Whereas previous studies on salivary gland extracts from the sandfly Lutzomyia longipalpis identified SALO (salivary anticomplement from L. longipalpis) as a potent inhibitor of the classical complement pathway (CP), its precise mechanism of action has remained elusive. We found that SALO inhibits the CP by binding specifically to the zymogen form of C1r. We provide two crystal structure determinations and supporting functional studies which show that SALO binds tightly to the zymogen activation loop of C1r preventing cleavage of its scissile bond. However, since the C1r zymogen undergoes autoactivation over time, we expressed an engineered fragment of human C1r consisting of its two CCP repeats and its serine protease domain, wherein the catalytic serine (S654) had been mutated to alanine (zC1r-12SP).

Thereafter, we crystallized eSALO-WT bound to zC1r-12SP, collected X-ray diffraction data extending to 3.3 Å limiting resolution, and solved the structure by molecular replacement. The asymmetric unit of the crystal contained two copies of the eSALO-WT–zCr-12SP complex, which superimposed well upon each other (RMSD = 0.34 Å across 444 equivalent Cα positions); thus, our subsequent analyses focused on the eSALO-WT–zC1r-12SP complex represented by chains A and C. Whereas the eSALO-WT–zC1r-12SP interaction buried ∼1100 Å2 of surface area at the interface, the most extensive interactions between the two proteins were centered upon the zymogen activation loop of zC1r-12SP. By contrast, there were no contacts between eSALO-WT and either of the CCP domains of the protease, which may be less accessible within the context of the larger C1 structure. Consistent with this, EBI-PISA identified 13 likely hydrogen bonds and four candidate salt bridges between the residues lining this channel, including N33 and Y/X51 (explained further in the following subsection), and residues from the zymogen activation loop of zC1r-12SP, which is composed roughly of residues V458-Q468 inclusive. At the periphery of the eSALO-WT channel, the side chain of E58 formed a salt bridge with the side chain of R461 from zC1r-12SP. Finally, outside the concave channel, residues on the first α helix of eSALO-WT, including D32, appeared to contact a secondary site on zC1r-12SP, which is composed of residues H642–Q647 inclusive. During the course of model building and refinement, we noticed a strong, positive feature in the Fo–Fc electron density map distal to the hydroxyl group of eSALO-WT residue Y51. Based on the geometry of this electron density, we suspected that Y51 had undergone post-translational sulfation during eSALO-WT expression and secretion from HEK293(T) cells. Therefore, we subsequently modeled this residue as sulfotyrosine, X51. In the final model, this sulfate group formed three different hydrogen bonds ranging from 2.6 to 3.2 Å in length with groups derived from R463 and I464, which are the two residues linked by the scissile bond in the C1r zymogen.

>SEDCENIFHDNAYLLKLDCEAGRVDPVEYDDISDEEIYEITVDVGVSSEDQEKVAKIIRECIAQVSTQDCTKFSEIYDCYMKKKICNYYPENMGSGHHHHHHHH[2x];>KCPQPKTLDEFTIIQNLQPQYQFRDYFIATCKQGYQLIEGNQVLHSFTAVCQDDGTWHRAMPRCKIKDCGQPRNLPNGDFRYTTTMGVNTYKARIQYYCHEPYYKMQTRAGSRESEQGVYTCTAQGIWKNEQKGEKIPRCLPVCGKPVNPVEQRQRIIGGQKAKMGNFPWQVFTNIHGRGGGALLGDRWILTAAHTLYPKEHEAQSNASLDVFLGHTNVEELMKLGNHPIRRVSVHPDYRQDESYNFEGDIALLELENSVTLGPNLLPICLPDNDTFYDLGLMGYVSGFGVMEEKIAHDLRFVRLPVANPQACENWLRGKNRMDVFSQNMFCAGHPSLKQDACQGDAGGVFAVRDPNTDRWVATGIVSWGIGCSRGYGFYTKVLNYVDWIKKEMEEEDGSGHHHHHHHH[2x]>[2x]SDEVRKNLMDMFRDRQAFSEHTWKMLLSVCRSWAAWCKLNNRKWFPAEPEDVRDYLLYLQARGLAVKTIQQHLGQLNMLHRRSGLPRPSDSNAVSLVMRRIRKENVDAGERAKQALAFERTDFDQ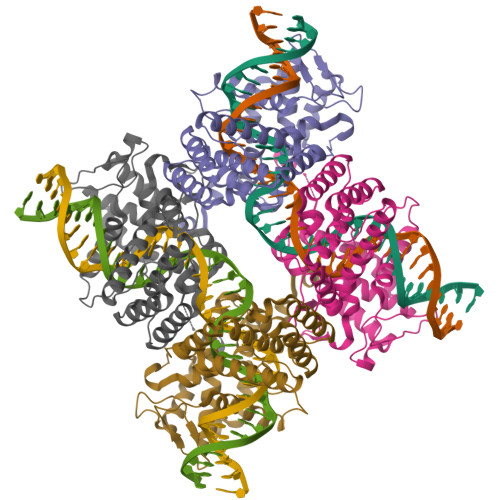VRSLMENSDRCQDIRNLAFLGIAYNTLLRIAEIARIRVKDISRTDGGRMLIHIGRTKTLVSTAGVEKALSLGVTKLVERWISVSGVADDPNNYLFCRVRKNGVAAPSATSQLSTRALEGIFEATHRLIYGAKDDSGQRYLAWSGHSARVGAARDMARAGVSIPEIMQAGGWTNVNIVMNYIRNLDSETGAMVRLLED The SALM family of proteins also known as LRR and fibronectin III domain containing proteins (LRFNs), represent a family of LRR-containing synaptic adhesion molecules, with five known members (SALM1-SALM5). SALMs are considered to be postsynaptic adhesion proteins, mostly expressed in the neurons and regulate neurite outgrowth and branching. SALM3 interacts with all three known members of LAR-RPTPs (LAR, PTPσ and PTPδ) to induce presynaptic differentiation. In this study, we have solved the crystal structure of mouse SALM3 LRR domain and show that it forms a dimer that is close to identical to that of SALM5, and the residues that are involved in dimerization and their interactions are largely conserved, and our complementary biophysical studies support this.

The structure of mouse SALM3 LRR domain was solved at 2.8 Å resolution in space group P21. Four molecules, or two dimers, were present in the asymmetric unit of the crystal, one monomer had an N-glycan partly visible in electron density at Asn25 at the N-terminal end of the domain. The LRR domain further contains an N-terminal LRRNT capping subdomain (residues 17–48) and an α-helical C-terminal LRRCT capping domain (residues 228–278), which are conserved in the vertebrate extracellular LRR domain family. Both the LRRNT and LRRCT subdomains of SALM3 are stabilized by two disulphide bridges; in the LRRNT between Cys17-Cys27 and Cys21-Cys34, and in the LRRCT between Cys238–Cys257 and Cys240-Cys278. A flexible loop (residues 216–227) is present between the 7th LRR and the LRRCT, not visible in the SALM3 crystal structure. The SALM3 LRR domain, like SALM5 and SALM2 forms an antiparallel side-by-side dimer, with a rather small interface with buried surface area of 1,001 Å2. The interface consists of the “one-layer” central hydrogen bonding network described above, and hydrophobic interactions formed by the N- and C-terminal regions. The hydrophobic interactions and hydrogen bonding networks are conserved at the interface with Gln131 and Arg107 forming hydrogen bonds across the dimer interface to Asn156 of the other monomer and vice versa. Comparison of the SALM3, SALM5 as well as SALM2 dimers reveals highly similar structures with r.m.s.d. values of 0.691 and 0.758 Å for the LRR domains of SALM5 and SALM2 against SALM3 structure, respectively. Thus, these measurements verified that the LRR domain is sufficient alone for stable dimer formation.

>MPLLLLLPLLWAGALAMDKLCPLPCVCQNLSESLSTLCAHRGLLFVPPNVDRRTVELRLADNFIQALGPPDFRNMTGLVDLTLSRNAITRIGARSFGDLESLRSLHLDGNRLVELGSSSLRGPVNLQHLILSGNQLGRIAPGAFDDFLDSLEDLDVSYNNLRQVPWAGIGSMPALHTLNLDHNLIDALPPGVFAQLSQLSRLDLTSNRLATLAPDPLFSRGRDAEASPSPLVLSFSGNPLHCNCELLWLRRLARPDDLETCASPPTLAGRYFWAVPEGEFSCEPPLIAGTRGSLEVLFQ[4x]> MNA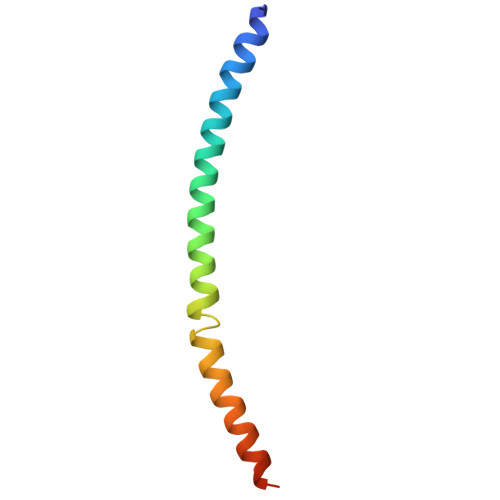NKQRQYNQLAHELRELQTNLQETTKQLDIMSKQCNENLVGQLGKVHGSWLIGSYIYYMEQMLGKTQ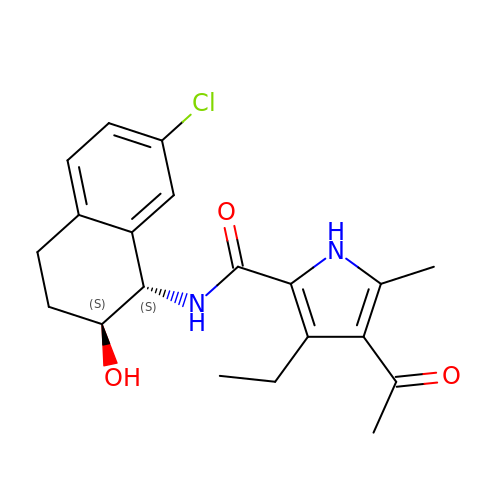~{N}-[(1~{S},2~{S})-7-chloranyl-2-oxidanyl-1,2,3,4-tetrahydronaphthalen-1-yl]-4-ethanoyl-3-ethyl-5-methyl-1~{H}-pyrrole-2-carboxamide | C20 H23 Cl N2 O3 | KVJAGYRUNZONPJ-WMZOPIPTSA-N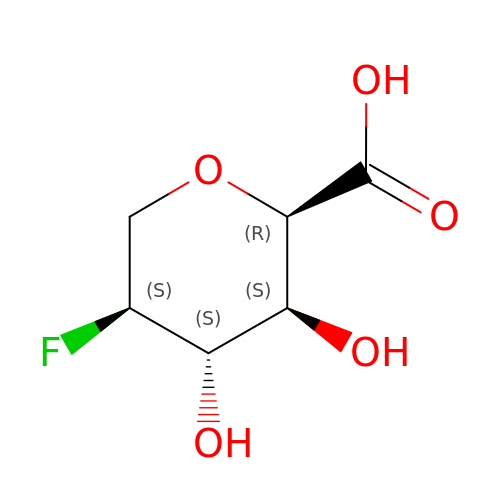2,6-anhydro-5-deoxy-5-fluoro-L-idonic acid | C6 H9 F O5 | KRAJNEOUENOZDR-SKNVOMKLSA-N N6-methyladenosine (m6A) is the most abundant and prevalent internal modification in mRNA. In mammals, m6A exerts pivotal roles in posttranscriptional regulation and its dysregulation is implicated in various diseases including cancer. m6A is installed by a multicomponent methyltransferase complex (MTC, also known as the m6A writer complex). The mammalian MTC is composed of the core m6A methyltransferase METTL3–METTL14 complex (MTC core) and several regulatory proteins including WTAP, the adaptor responsible for METTL3–METTL14 localization and proper substrate recruitment, and VIRMA (KIAA1429), the specificity mediator that mediates preferential m6A modification at the 3′ untranslated regions (UTRs). WTAP and VIRMA are important subunits of the m6A writer complex.

In parallel, we obtained the WTAP protein alone (residues 130–241, WTAP130–241) using the Escherichia coli expression system and determined the crystal structure of the WTAP (2.40 Å). Two molecules of WTAP (with the assigned density of residues 150–241, WTAP150–241) formed a symmetric parallel α-helical coiled-coil homodimer through hydrophobic interactions between two identical surface patches. Specifically, the side chains of residues M158, I165, L183, L204, I208, L211, V215, M218, I222, L225, L229 and L236 from the two WTAPs formed a hydrophobic interaction network. The structure of the asymmetric WTAP171–237 dimer in the quaternary complex is similar to the crystal structure of the symmetric WTAP150–241 dimer with a root-mean-square deviation (RMSD) of 4.2 Å over 134 Cα atoms. However, compared to the WTAPs alone, VIRMA-bound WTAPs bent around the observed N-termini (around WTAPA residue 188 and WTAPB residue 185) and displayed a more compact and dense conformation with distinct intramolecular interactions.

>[2x]QTKDKLEQAQNELSAWKFTPDSQTGKKLMAKCRMLIQENQELGRQLSQGRIAQLEAELALQKKYSEELKSSQDELNDFIIQLDEEVEGMQSTILVLQQQLKETRQQLAQYQQLEHHHHHHHH Sequence alignment revealed that Vps75 is a member of the evolutionarily conserved nucleosome assembly protein 1/SE translocation (NAP1/SET) superfamily, members of which function as escorts for histone (H3–H4)2 tetramers and H2A–H2B dimers. Two histone chaperones, Vacuolar Protein Sorting 75 (Vps75) and the Anti-Silencing Function 1 protein (Asf1), are involved in the Rtt109-dependent histone H3K9, H3K27, and H3K56 acetylation. In this study, we solved both dimeric and tetrameric structures of Vps75 from a pathogenic fungus, P. carinii (PcVps75), and identified a structural basis for the inability of PcVps75 to interact with PcRtt109. Therefore, we propose that Vps75 regulates the HAT activity of Rtt109 by affecting the interactions between histones and specific histone chaperones rather than by forming a complex with Rtt109.

The PcVps75 dimer adopts a classic “head-phone” topology, which is characteristic of the NAP family. The PcVps75 protomer contains two major structural domains, a long α-helix at the N terminus (domain I, residues 18–58, colored green) and a α + β globular domain (domain II, residues 64–221, colored orange). An acidic disordered region (residues 224–250) at the C terminus is truncated owing to its flexibility. Two major histone-binding surfaces were identified for the PcVps75 dimer, including the disordered C-terminal tail and a highly negatively charged region that included residues E192, D193, E194, E195, E196, E203, and D204. Within α helix α7 of PcVps75, a highly negatively charged region that includes E192, D193, E194, E195, E196, E203, and D204 may mediate interactions with histones. Similar to many histone chaperones, PcVps75 contains a long, disordered tail of acidic amino acids that interacts with basic histones, leading to charge neutralization. However, the interaction between PcVps75∆C-K5 and histones is completely abolished. Finally, we revealed that helix α7, which is located within the highly acidic concave surface of PcVps75, and the CTAD domain are both necessary for PcVps75 to interact with histones. We also noticed that the PcVps75 dimer is much more stable in a homogeneous state than tetrameric Vps75 in vitro.

>[2x]MSAKKTNEKRSEIQSETNTTSLDEVADIELEFEKADVELLKHQVELFNPLYEKRANVLRKIPKFWPIAIEAAPSDELSVYISPEDANVLEHLIDLRVYRPNEDPRDIKIVFEFEANEYLESNSLYLEKLFRYSSQKAEASSSNINKEPSQLISEKVNIEWKKNKDLTRQTKGTAPSFFTWFSWTGKENDIFEDEEELAIFIAEDLYPNAVKYFTDALQENEENEDEEIDLENENGDNISEEEPSKKRTKL> NSLNAIEEPVTRRHHQRHHEREREENGYCAPYSGKVCKEYLTGQVWYSLEDPTGGWKNEQVTTALWDELISDLTGLCREAAEKMLCAYAFPNCHMEGGRAVKAPLCFEDCQATHLQFCYNDWVLIEEKKERNMFIKSRGHFRLPNCSSLPHYNASM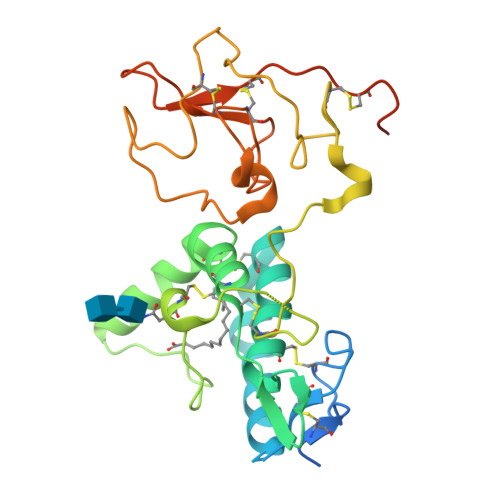RRPNCSYIGLTELKESEVSYDCRNGNGRFYMGTMNVSKSGIPCQRWDTQYPHKHFQPPLVFHQLLEGENYCRNAGGEEPHPWCYTVDESVRWQHCDIPMCPDYVDPNAVDLNTPIKMEKFFTPS>[2x]SETRLSLEDLFRKDFVLHDPEARWINDTDVVYKSENGHVIKLNIETNATTLLLENTTFVTFKASRHSVSPDLKYVLLAYDVKQIFHYSYTASYVIYNIHTREVWELNPPEVEDSVLQYAAWGVQGQQLIYIFENNIYYQPDIKSSSLRLTSSGKEEIIFNGIADWLYEEELLHSHIAHWWSPDGERLAFLMINDSLVPTMVIPRFTGALYPKGKQYPYPKAGQMNPTIKLYVVNLYGPTHTLELMPPDSFKSREYYITMVKWVSNTKTVVRWLNRAQNISILTVCETTTGACSKKYEMTSDTWLSQQNEEPVFSRDGSKFFMTVPVKQGGRGEFHHIAMFLIQSKSEQ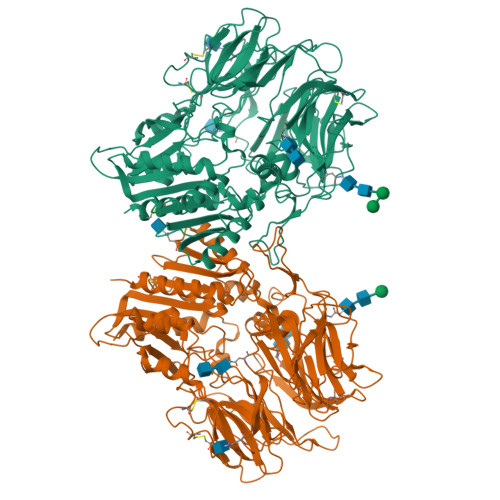ITVRHLTSGNWEVIKILAYDETTQKIYFLSTESSPRGRQLYSASTEGLLNRQCISCNFMKEQCTYFDASFSPMNQHFLLFCEGPRVPVVSLHSTDNPAKYFILESNSMLKEAILKKKIGKPEIKILHIDDYELPLQLSLPKDFMDRNQYALLLIMDEEPGGQLVTDKFHIDWDSVLIDMDNVIVARFDGRGSGFQGLKILQEIHRRLGSVEVKDQITAVKFLLKLPYIDSKRLSIFGKGYGGYIASMILKSDEKLFKCGSVVAPITDLKLYASAFSERYLGMPSKEESTYQAASVLHNVHGLKEENILIIHGTADTKVHFQHSAELIKHLIKAGVNYTMQVYPDEGHNVSEKSKYHLYSTILKFFSDCLKE> MSRIRTSLEVLSLGFGLFTAEALYSGNEHFYKDWFLPTARLLVRDGE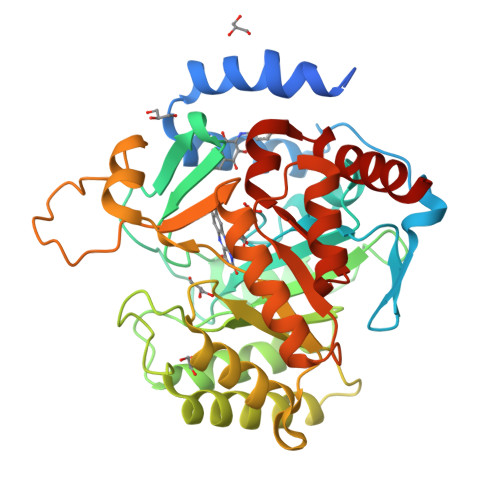TAHNLSVYLASYGFIPHKQRNSFPQLKCKVFGLEFDHPIGLAAGFDKDGKAFMGLLNAGFSHIEVGTVTPNPQLGNARPRIFRWTEKEAVVNRCGFNSDGHDAVYERLKDRPWEGRGVIGVNLGCNKTSADPTADYVAGVRKFGEVADYLVINVSSPNTPGLRSLQTKEKLRDLLSKVLAARNQLSKKTPILLKISPDENDQNLKDIVEVALDSKTRIDGMIISNTTLTTYEEAVACGAAPIPGNNKQNVVYGGLSGRPLFEKSTDCLRKVSALTKGAIPLIGVGGISCGEDALSKLNAGASLVQLYTSFVYQGPPVAHKVAREINKLKMTS> MDVSGQETDWRSAAFRQKLVSQIEDAMRKAGVAHSKSSKDMESHVFLKAKTRDEYLSLVARLIIHFRDIHNKKSQASVSDPMNALQSLTGGPTPGAAGIGMPPRGPGQSLGGMGGLGAMGQPLPLSGQPPPGTSGMAPHGMAVVSTATPQTQLQLQQVALQQQQQQQQQQQFQQQQAALQQQQQQQQQQQQQQQFQAQQNAMQQQFQAVVQQQQLQQQQQQQHLIKLHHQSQQQQIQQQQLQRMAQLQLQQQQQQQQQQALQAQPPMQQPSMQQPQPPPSQALPQQLSQLHHPQHHQPPPQAQQSPIAQNQPPQIPPQSQSQPLVSQAQALPGPMLYAAQQQLKFVRAPMVVQQPQVQPQVQQVQPQVQPQAAVQAAQSAQMVAPGVQMIAEALAQGGMHVRARFPPTSTMSAGPSSSISLGGQPTTQVSQSSLTMLSSPSPGQQVQTPQSMPPPPQPSPQPGSQPNSNVSSGPAPSPSSFLPSPSPQPSQSPVTARTPQNFSVPSPGPLNTPVNPSSVMSPAGSSQAEEQQYLDKLKQLSKYI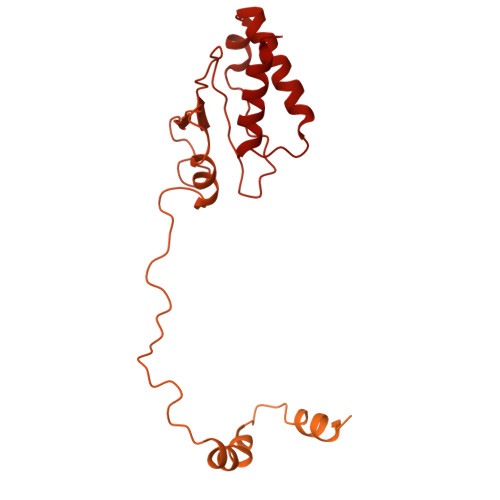EPLRRMINKIDKNEDRKKDLSKMKSLLDILTDPSKRCPLKTLQKCEIALEKLKNDMAVPTPPPPPVLPTKQQDLCQPLLDAVLANIRSPVFNHSLYRTFVPAMMAIHGPPIVSPVVCSRKRRFEEDERQSIPNVLQGEVARLDPKFLVNLDPSHCSNNGTVHLICKLDDKDLPSVPPLELSVPADYPAQSPMWIDRQWQYDANPFLQSVHRCMTSRLLQLPDKHSVTALLNTWAQSIHQACLSAA> 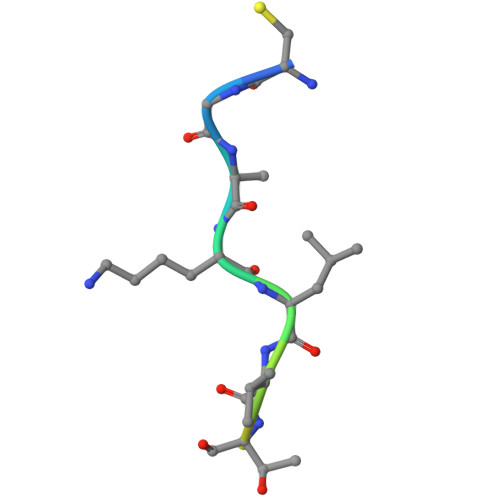CGKKLVTQEVSPK>ASGNARIGKPAPDFKATAVVDGAFKEVKLSDYKGKYVVLFFYPLDFTFVCPT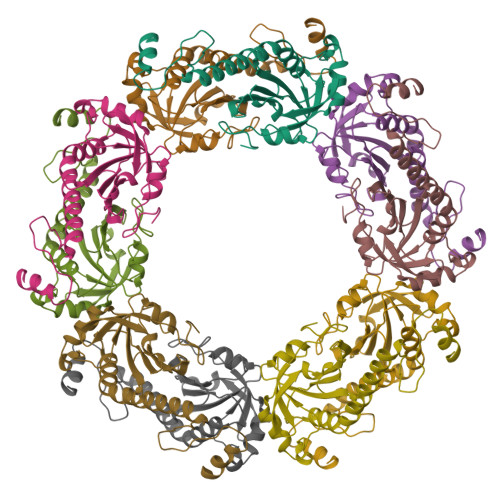EIIAFSNRAEDFRKLGCEVLGVSVDSQFTHLAWINTPRKEGGLGPLNIPLLADVTRRLSEDYGVLKTDEGIAYRGLFIIDGKGVLRQITVNDLPVGRSVDEALRLVQAFQYTDEHGEVCPAGWKPGSDTIKPNVDDSKEYFSKHN[10x]> HAASRPNIILVMADDLGIGDPGCYGNKTIRTPNIDRLASGGVKLTQHLAASPLATPSRAAFMTGRYPVRSGMASWSRTGVFLFTASSGGLPTDEITFAKLLKDQGYSTALIGKWHLGMSCHSKTDFCHHPLHHGFNYFYGISLTNLRDCKPGEGSVFTTGFKRLVFLPLQIVGVTLLT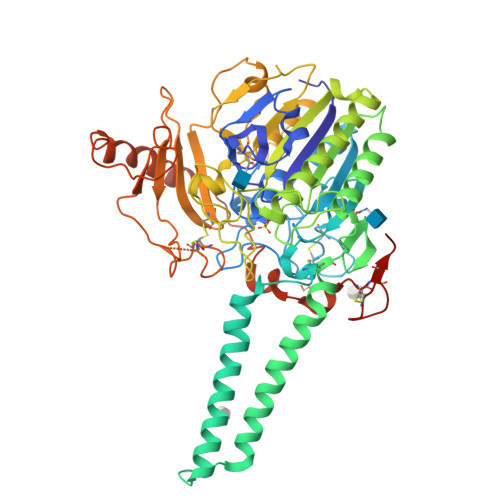LAALNCLGLLHVPLGVFFSLLFLAALILTLFLGFLHYFRPLNCFMMRNYEIIQQPMSYDNLTQRLTVEAAQFIQRNTETPFLLVLSYLHVHTALFSSKDFAGKSQHGVYGDAVEEMDWSVGQILNLLDELRLANDTLIYFTSDQGAHVEEVSSKGEIHGGSNGIYKGGKANNWEGGIRVPGILRWPRVIQAGQKIDEPTSNMDIFPTVAKLAGAPLPEDRIIDGRDLMPLLEGKSQRSDHEFLFHYCNAYLNAVRWHPQNSTSIWKAFFFTPNFNPVGSNGCFATHVCFCFGSYVTHHDPPLLFDISKDPRERNPLTPASEPRFYEILKVMQEAADRHTQTLPEVPDQFSWNNFLWKPWLQLCCPSTGLSCQCDREKQDKRLSR>YVEGQRKRRNTIHEFKKSAKTTLIKIDPALKIKTKKVNTADQCANRCTRNKGLPFTCKAFVFDKARKQCLWFPFNSMS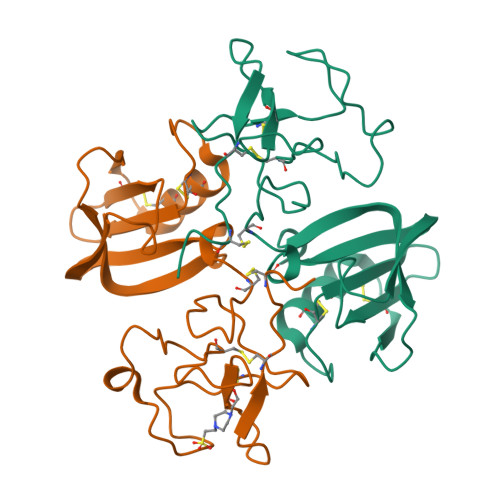SGVKKEFGHEFDLYENKDYIRNCIIGKGRSYKGTVSITKSGIKCQPWSSMIPHEHSFLPSSYRGKDLQENYCRNPRGEEGGPWCFTSNPEVRYEVCDIPQCSEVE[2x]>[2x]GSMKQIYDTLQLIPVDKIDLHEAFEPSRLEKTKESIAKEQHLRHPVLVVKTLFGRYMVIDGVHRFMSLKALGCEVIPVQVIQRTQYSIGSWHHKIPNGAWCEGLTDEELLPWTTEVRDETPFITMCDQQTEHYLYVADLTVDKLDIWKKVVNSYSASCNVERVPHSACLCLDSNDILMKYQPLQIGEIEAVVQRGQTVPAGVTRFNIAGRCLNLQVPLHLLKNSNLGNQEQWHTF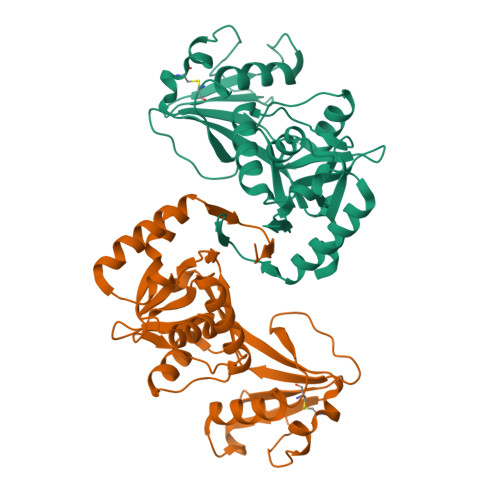LQKKIESMRCYTEKIYLIEAE> MRGSHHHHHHGMASNEFPVVLVINCGSSSIKFSVLDVATCDVLMAGIADGMNTENAFLSINGDKPINLAHSNYEDALKAIAFELEKRDLTDSVALIGHRIAHGGELFTQSVIITDEIIDNIRRVSPLAPLHNYANLSGIDAARHLFPAVRQVAVFDTSFHQTLAPEAYLYGLPWEYFSSLGVR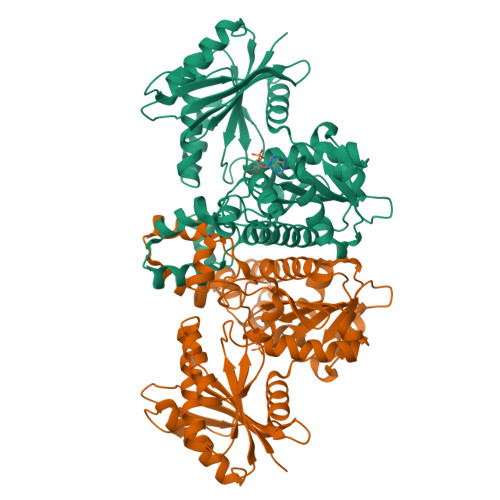RYGFHGTSHRYVSRRAYELLDLDEKDSGLIVAHLGNGASICAVRNGQSVDTSMGMTPLEGLMMGTRSGDVDFGAMAWIAKETGQTLSDLERVVNKESGLLGISGLSSDLRVLEKAWHEGHERARLAIKTFVHRIARHIAGHAASLHRLDGIIFTGGIGENSVLIRQLVIEHLGVLGLTLDVEMNKQPNSHGERIISANPSQVICAVIPTNEEKMIALDAIHLGNVKAPVEFA>[6x]MQQNFGTALGDGFVLNEATLMIGALGSALDLTEEEHSVGLFKNLAIANDKTFQDLNQGVTQDTVHSQKTGDNWTISGNGYEYNPRTIMYALGQAGFTADPTAARTRAVVSAPAAVGVSEISVQSATGLAVGDWVILYNKLGDNNGLAYKIDAIATNTITLDRDLVAPVAVGDELVKSTLINTNNPNSCSGAEYFSAKIVSADVNCNPIVV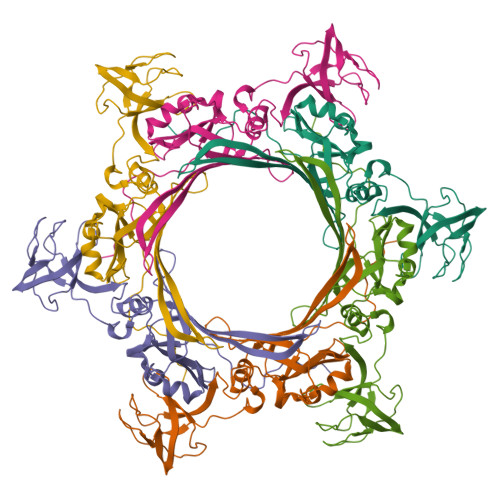IVPKVQITSGLNLAFGATDYANIAYQMKAMALTRKDAGYDLYVQHGKSKVFLLT> GSMANIAVQRIKREFKEVLKSEETSKNQIKVDLVDENFTELRGEIAGPPDTP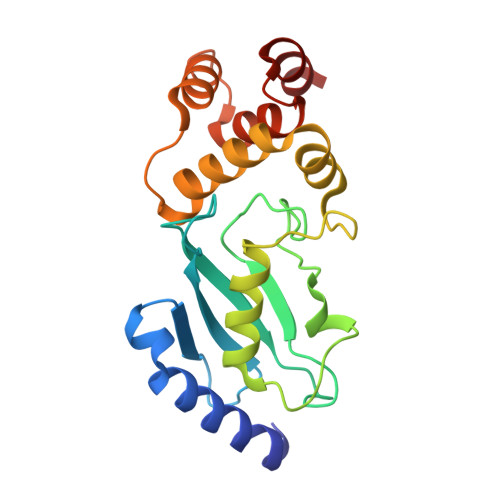YEGGRYQLEIKIPETYPFNPPKVRFITKIWHPNISSVTGAICLDILKDQWAAAMTLRTVLLSLQALLAAAEPDDPQDAVVANQYKQNPEMFKQTARLWAHVYAGAPVSSPEYTKKIENLCAMGFDRNAVIVALSSKSWDVETATELLLSN>MKPYDLSEAVAVVTGGSSGIGLATVELLLEAGAAVAFCARDGERLRAAESALRQRFPGARLFASVCDVLDALQVRAFAEACERTLGCASILVNNAGQGRVSTFAETTDEA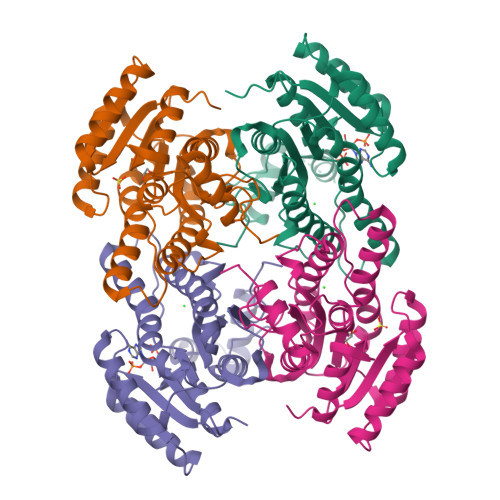WSEELQLKFFSVIHPVRAFLPQLESRADAAIVCVNSLLASQPEPHMVATSAARAGVKNLVRSMAFEFAPKGVRVNGILIGLVESGQWRRRFEAREERELDWAQWTAQLARNKQIPLGRLGKPIEAARAILFLASPLSAYTTGSHIDVSGGLSRHA[4x]>MSEKKEARVVINDLLAEQYANAFKAKEEGRPVGWSTSVFPQELAEVFDLNVLYPENQAAGVAAKKGSLELCEIAESKGYSIDLCAYARTNFGLLENGGCEALDMPAPDFLLCCNNICNQVIKWYENISRELDIPLIMIDTTFNNEDEVTQSRIDYIKAQFEEAIKQLEIISGKKFDPKKFEEVMKISAENGRLWKYSMSLPADSSPSPMNGFDLFTYMAVIVCARGKKETTEAFKLLIEELEDNMKTGKSSFRGEEKYRIMMEGIPCWPYIGYKMKTLAKFGVNMTGSVYPHAWALQYEVNDLDGMAVAYSTMFNNVNLDRMTKYRVDSLVEGKCDGAFYHMNRSCKLMSLIQYEMQRRAAEETGLPYAGFDGDQADPRAFTNAQF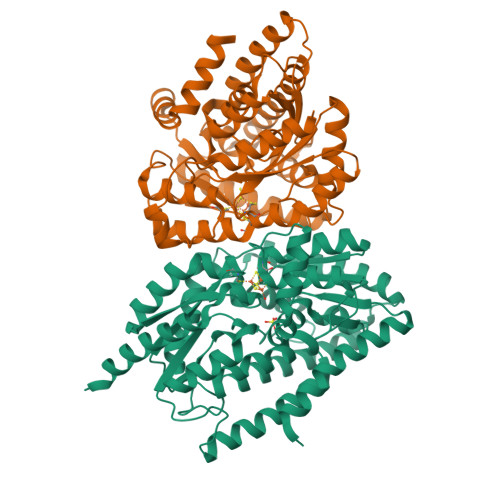ETRIQGLVEVMEERKKLNRGEI[2x];>[2x]MEAILSKMKEVVENPNAAVKKYKSETGKKAIGCFPVYCPEEIIHAAGMLPVGIWGGQTELDLAKQYFPAFACSIMQSCLEYGLKGAYDELSGVIIPGMCDTLICLGQNWKSAVPHIKYISLVHPQNRKLEAGVKYLISEYKGVKRELEEICGYEIEEAKIHESIEVYNEHRKTMRDFVEVAYKHSNTIKPSIRSLVIKSGFFMRKEEHTELVKDLIAKLNAMPEEVCSGKKVLLTGILADSKDILDILEDNNISVVADDLAQETRQFRTDVPAGDDALERLARQWSNIEGCSLAYDPKKKRGSLIVDEVKKKDIDGVIFCMMKFCDPEEYDYPLVRKDIEDSGIPTLYVEIDQQTQNNEQARTRIQTFAEMMSLASAWSHPQFEK> MNEKTMQIEQIVKKVKECSLTPEEGLELIKSLGKTHLYEMVWDRHEFKGSKKFPHTKEPILFFCEDDSMYTVMKRQLEGYEAPFIYVTSGERFEDCRNGRFTMNFTKGEDYDALCGVLRSQNIRPRHIIHFLAAGLFKNTEDAMRKQLNKSLYSLFQMFQAFMANKLCPKAEILYLYENAEGEVQPIYNAVESFLKTVQAENPNFTCKAAELKSMFDEPFTKQHIADVISFEWNNQCKTDCFTCYEPRHYYKRQLQRVKKEDGEKHSFSVKKNGVYLITGGAGGLGYLFAEYLAKQAEVKLILTGRSPASRETAQKLSALENLGAEALYVPADISKEKETDALIKYIKQTFGELNGILHSAGLVKDAFIIKKTKESIEEVIAPKVFGT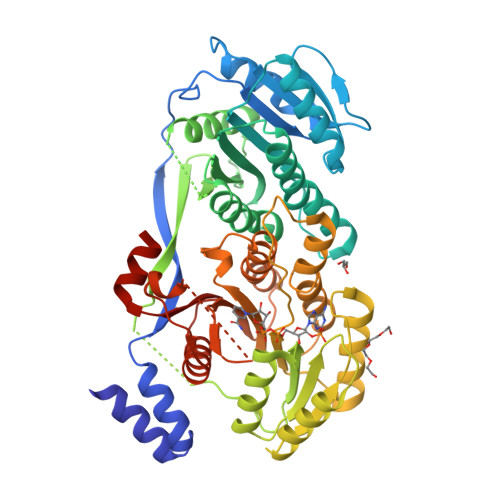VWLDKAAEEEPLDFFVMFSSLSAVLPNAGQSDYAFANGCMDGFTQYRSMKGRPGKTLSINWPLWDAGNMTVGPGELQALRHAGLELLSAQAGLAAFQDSMSRSASQLAVISGDKDRISELLSTDHKKIETVPEN> MGSHHHHHHSSGLVPRGSHMSEPQRLKPVFP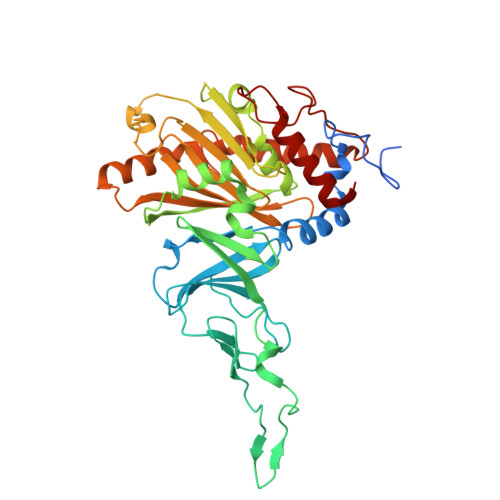QDPKWPGEGSSRVPFWAYTREDLYKRELERLFYANHWCYVGLEAEIPNPGDFKRTVIGERSVIMVRDPDGGINVVENVCAHRGMRFCRERHGNAKDFFCPYHQWNYSLKGDLQGVPFRRGVKQDGKVNGGMPKDFKLEEHGLTKLKVAARGGAVFASFDHDVEPFEEFLGPTILHYFDRVFNGRKLKILGYRRQRIPGNWKLMQENIKDPYHPGLLHTWFSTFGLWRADNKSELKMDAKFRHAAMISTRGQGGKNEEVVSGVDSFKEQMKVNDPRLLDIVPEPWWGGPTAVMTTIFPSVIIQQQVNSVSTRHIQPNGHGSFDFVWTHFGFEDDNEEWTQRRLIQANLFGPAGFVSADDGEVIEWSQEGFEQKPTHRTVIEMGGHEIGDTDHMVTETLIRGMYDYWRKVMGE> MRKNFKAFVALFAAILLFFSGCSSKQEAKAPKSEVIYQVMVDRFYNGDPSNDDPEVSKGMFDPTHTNWRMYWGGDLKGLTEKIPYIKGMGVTAIWISPVVDNINKPAVYNGEINAPYHGYWARDFKRVEEHFGTWEDFDNFVKVAHENGIKVILDFAPNHTSPADEENPDFAENGALYDDGKLLGTYSNDSLKLFHHNGSISNWNNLKELQDKNLFDLADLDQSNPIVDKYLKDSIKLWFNHEIDGVRLDAAKHMPMEWVKSFANTIYSIKKDVLLFGEWMLSGPTDPLYGYNIQFANTTGFSVLDFMLNGAIRDVFGKGYGFERLNDTLEDTNKDYENPYKLVTFIDNHDMPRFLSLNNDKDKLHEAIAFIMTTRGIPVIYYGTEQYLHNDTNGGNDPYNRPMMEKFDESTKAYTLIKELSRLRQLTPALQYGTTTARYVSDDVYIYERQYGKDVVLVAINKGEKTTVKTVKTSLRKGIYKDYLKGLLKGVELKVTKGNGENLVQDLTLPGNSVSVWTNVRVKA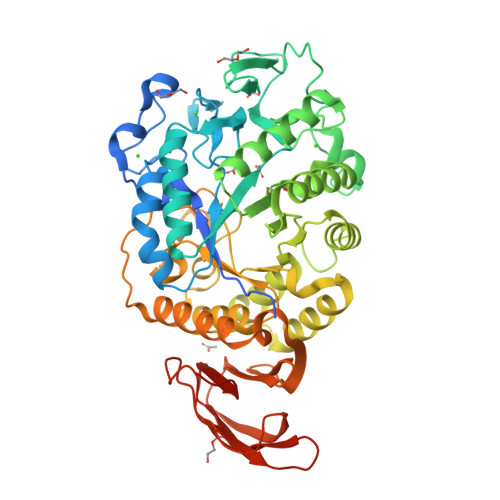AALEHHHHHH>[5x]MALLLASAINHTAHPAGLRSHPNNESFSRHHLCSSPQNISKRRSNLSFRPRAQTISSESAGIHRLSPWEIPRRDWFPPSFLFGAATSAYQIEGAWNEDGKGPSTWDHFCHNFPEWIVDRSNGDVAADSYHMYAEDVRLLKEMGMDAYRFSISWPRILPKGTLAGGINEKRVEYYNKLIDLLLENGIEPYITIFHWDTPQALVDAYGGFLDERIIKDYTDFAKVCFEKFGKTVKNWLTFNEPETFCSVSYGTGVLAPGRCSPGVSCAVPTGNSLSEPYIVAHNLLRAHAETVDIYNKYHKGADGRIGLALNVFGRVPYTNTFLDQQAQERSMDKCLGWFLEPVVRGDYPFSMRVSARDRVPYFKEKEQEKLVGSYDMIGINYYTSTFSKHIDLSPNNSPVLNTDDAYASQETKGPDGNAIGPPTGNAWINMYPKGLHDILMTMKNKYGNPPMYITENGMGDIDKGDLPKPVALED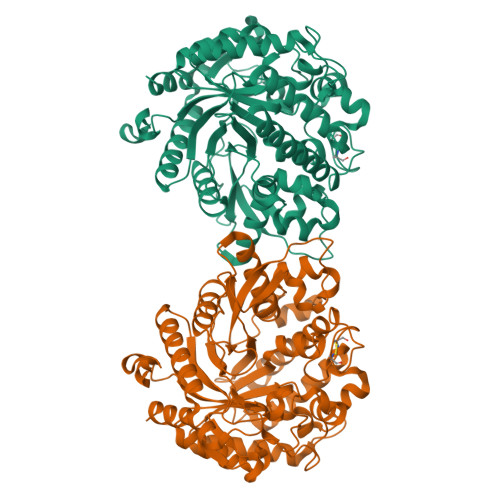HTRLDYIQRHLSVLKQSIDLGADVRGYFAWSLLDNFEWSSGYTERFGIVYVDRENGCERTMKRSARWLQEFNGAAKKVENNKILTPAGQLN;> MALLLASAINHTAHPAGLRSHPNNESFSRHHLCSSPQNISKRRSNLSFRPRAQTISSESAGIHRLSPWEIPRRDWFPPSFLFGAATSAYQIEGAWNEDGKGPSTWDHFCHNFPEWIVDRSNGDVAADSYHMYAEDVRLLKEMGMDAYRFSISWPRILPKGTLAGGINEKRVEYYNKLIDLLLENGIEPYITIFHWDTPQALVDAYGGFLDERIIKDYTDFAKVCFEKFGKKVKNWLTFNEPETFCSVSYGTGVLAPGRCSPGVSCAVPTGNSLSEPYIVAHNLLRAHAETVDIYNKYHKGADGRIGLALNVFGRVPYTNTFLDQQAQERSMDKCLGWFLEPVVRGDYPFSMRVSARDRVPYFKEKEQEKLVGSYDMIGINYYTSTFSKHIDLSPNNSPVLNTDDAYASQETKGPDGNAIGPPTGNAWINMYPKGLHDILMTMKNKYGNPPMYITENGMGDIDKGDLPKPVALEDHTRLDYIQRHLSVLKQSIDLGADVRGYFAWSLLDNFEWSSGYTERFGIVYVDRENGCERTMKRSARWLQEFNGAAKKVENNKILTPAGQLN>[4x]MNSNKELMQRRSQAIPRGVGQIHPIFADRAENCRVWDVEGREYLDFAGGIAVLNTGHLHPKVVAAVEAQLKKLSHTCFQVLAYEPYLELCEIMNQKVPGDFAKKTLLVTTGSEAVENAVKIARAATKRSGTIAFSGAYHGRTHYTLALTGKVNPYSAGMGLMPGHVYRALYPCPLHGISEDDAIASIHRIFK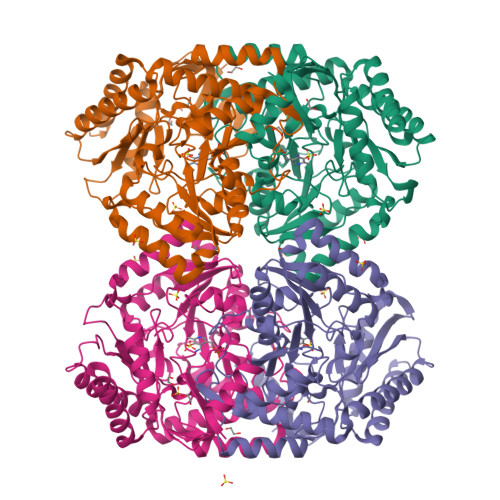NDAAPEDIAAIVIEPVQGSGGFYASSPAFMQRLRALCDEHGIMLIADEVQSGAGRTGTLFAMEQMGVAPDLTTFAKSIAGGFPLAGVTGRAEVMDAVAPGGLGGTYAGNPIACVAALEVLKVFEQENLLQKANDLGQKLKDGLLAIAEKHPEIGDVRGLGAMIAIELFEDGDHNKPDAKLTAEIVARARDKGLILLSCGPYYNVLRILVPLTIEDAQIRQGLEIISQCFDEAKQ>MEAVVISGRKLAQQIKQEVRQEVEEWVASGNKRPHLSVILVGENPASHSYVLNKTRAAAVVGINSETIMKPASISEEELLNLINKLNNDDNVDGLL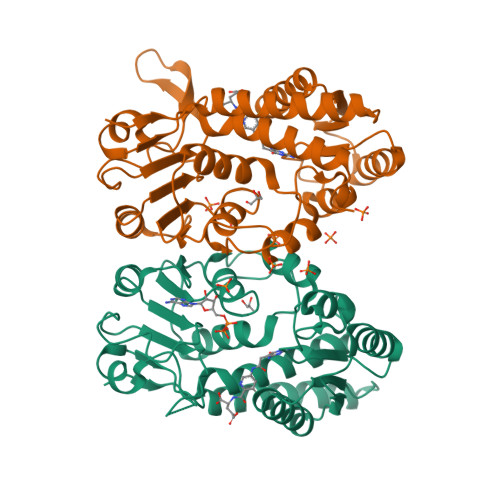VQLPLPEHIDERRICNAVSPDKDVDGFHVINVGRMCLDQYSMLPATPWGVWEIIKRTGIPTLGKNVVVAGRSKNVGMPIAMLLHTDGAHERPGGDATVTISHRYTPKEQLKKHTILADIVISAAGIPNLITADMIKEGAAVIDVGINRVHDPVTAKPKLVGDVDFEGVRQKAGYITPVPGGVGPMTVAMLMKNTIIAAKKVLRLEEREVLKSKELGVATN[2x]> APTSSSTKKTQLQLEHLLLDLQMILNGINNCKNPKLTRMLTFKFYMPKKATELKHLQCLEEELKPLEEVLNLAQSKNFHLRPRDLISNINVIVLELKGSETTFMC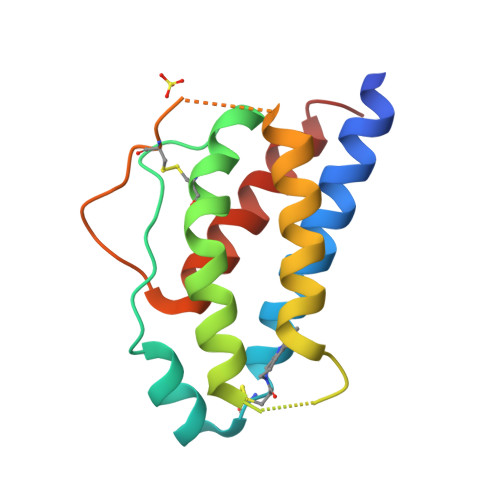EYADETATIVEFLNRWITFCQSIISTLT4-[4-(trifluoromethyl)phenyl]-1,2,3-thiadiazol-5-amine | C9 H6 F3 N3 S | 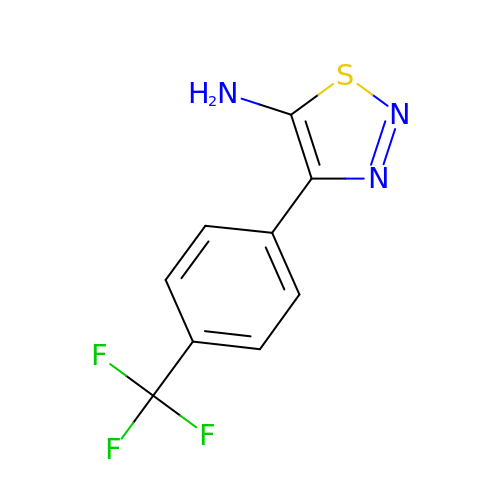URPRRYYGDXSCNR-UHFFFAOYSA-N>IRMVPISFVFNRFPRMVRDLAKKMNKEVNFIMRGEDTELDRTFVEEIGEPLLHLLRNAIDHGIEPKEERIAKGKPPIGTLILSARHEGNNVVIEVEDDGRGIDKEKIIRKAIEKGLIDESKAATLSDQEILNFLFVPGFSTKEKVSEVSGRGVGMDVVKNVVESLN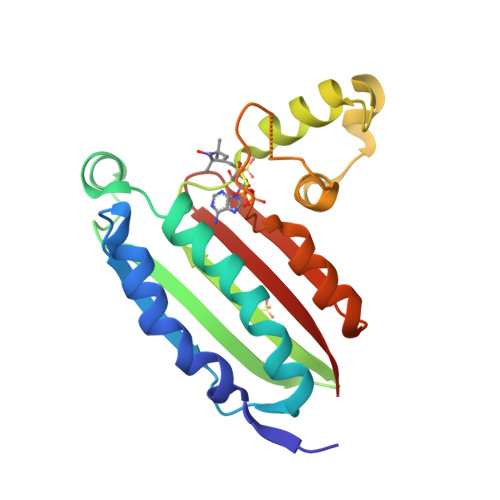GSISIESEKDKGTKVTIRLPL[4x]> MEEGFRDRAAFIRGAKDIAKEVKKHAAKKVVKGLDRVQDEYSRRSY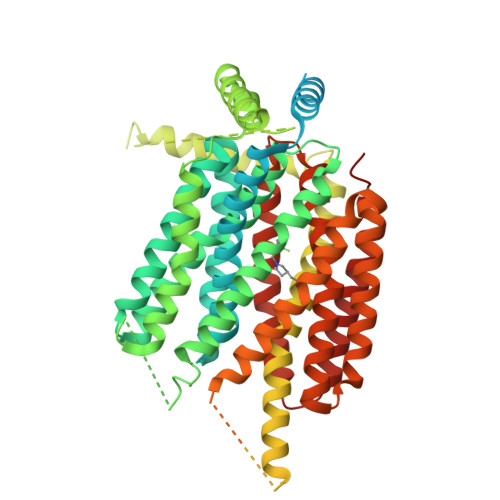SRFEEEDDDDDFPAPSDGYYRGEGTQDEEEGGASSDATEGHDEDDEIYEGEYQGIPRAESGGKGERMADGAPLAGVRGGLSDGEGPPGGRGEAQRRKEREELAQQYEAILRECGHGRFQWTLYFVLGLALMADGVEVFVVGFVLPSAEKDMCLSDSNKGMLGLIVYLGMMVGAFLWGGLADRLGRRQCLLISLSVNSVFAFFSSFVQGYGTFLFCRLLSGVGIGGSIPIVFSYFSEFLAQEKRGEHLSWLCMFWMIGGVYAAAMAWAIIPHYGWSFQMGSAYQFHSWRVFVLVCAFPSVFAIGALTTQPESPRFFLENGKHDEAWMVLKQVHDTNMRAKGHPERVFSVTHIKTIHQEDELIEIQSDTGTWYQRWGVRALSLGGQVWGNFLSCFGPEYRRITLMMMGVWFTMSFSYYGLTVWFPDMIRHLQAVDYASRTKVFPGERVEHVTFNFTLENQIHRGGQYFNDKFIGLRLKSVSFEDSLFEECYFEDVTSSNTFFRNCTFINTVFYNTDLFEYKFVNSRLINSTFLHNKEGCPLDVTGTGEGAYMVYFVSFLGTLAVLPGNIVSALLMDKIGRLRMLAGSSVMSCVSCFFLSFGNSESAMIALLCLFGGVSIASWNALDVLTVELYPSDKRTTAFGFLNALCKLAAVLGISIFTSFVGITKAAPILFASAALALGSSLALKLPETRGQVLQ> MAAGGAFVSEGGGGGRSYEGGVTAFVIMTCIVAAMGGLLFGYDLGISGGVTSMEEFLTKFFPQVESQMKKAKHDTAYCKFDNQMLQLFTSSLYLAALVASFMASVITRKHGRKVSMFIGGLAFLIGALFNAFAVNVSMLIIGRLLLGVGVGFANQSTPVYLSEMAPAKIRGALNIGFQMAITIGILVANLINYGTSKMAQHGWRVSLGLAAVPAVVMVIGSFILPDTPN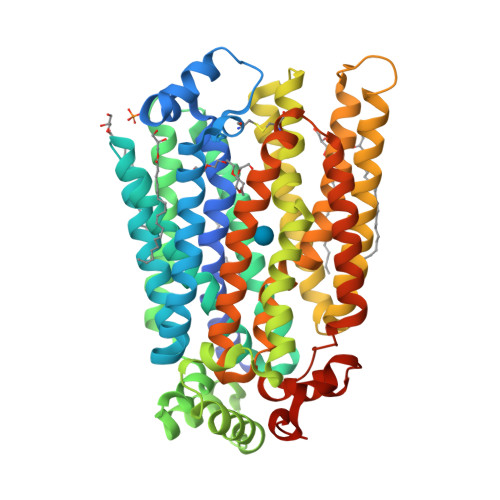SMLERGKNEEAKQMLKKIRGADNVDHEFQDLIDAVEAAKKVENPWKNIMESKYRPALIFCSAIPFFQQITGINVIMFYAPVLFKTLGFGDDAALMSAVITGVVNMLSTFVSIYAVDRYGRRLLFLEGGIQMFICQLLVGSFIGARFGTSGTGTLTPATADWILAFICVYVAGFAWSWGPLGWLVPSEICPLEIRPAGQAINVSVNMFFTFLIGQFFLTMLCHMKFGLFYFFASMVAIMTVFIYFLLPETKGVPIEEMGRVWKQHWFWKKYIPEDAIIGGHDDNNTNPGLVPR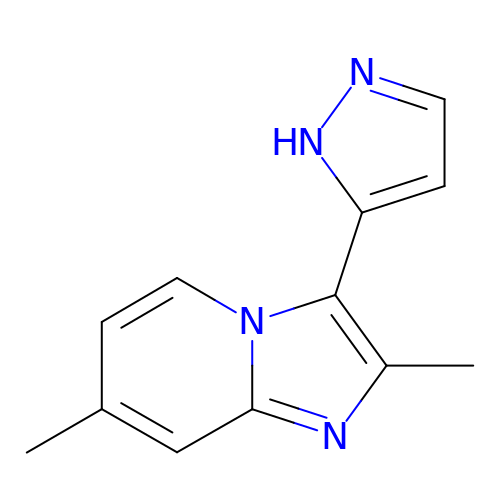2,7-dimethyl-3-(1H-pyrazol-5-yl)imidazo[1,2-a]pyridine | C12 H12 N4 | ZNRUSTFXUSPVPD-UHFFFAOYSA-N> GAMGNQEVNQNQRGKNKLLNDLRNLIEKANTDRKKYEKKLKEEPEDQYGILAFKSLRWHEEPRETVSDNSERSKAYRKLT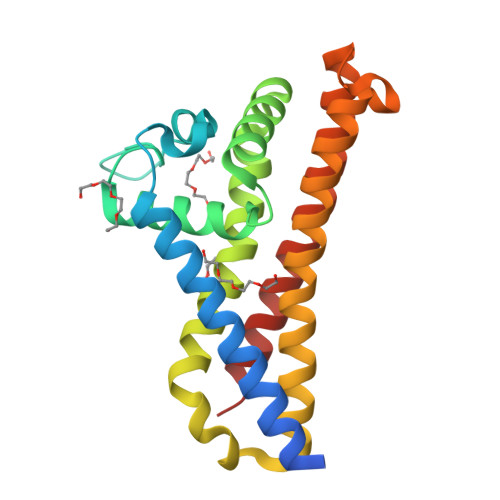YGILNDMNADELKRFSEIIILANEVEDIFNTSITLEGNIDYTIIHLYPKKDNLNKLKISDLENLKNLFEKLLSTKEIISKTFKQLLLDYQDDNNSIKADANKLKLHVKEIVKQIKEKQEESEKLKSDILSIKNF1-methyl-1H-pyrazol-4-amine | C4 H7 N3 | 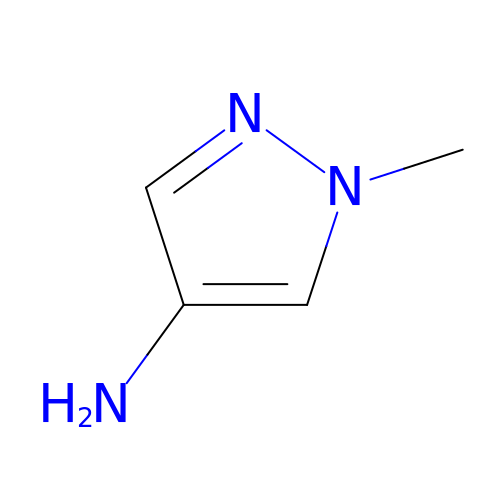LBGSWBJURUFGLR-UHFFFAOYSA-N>[6x]GSMPLLLDDGDPKAQTGFDLSTATTLFWRPVPVHVKQQDREDV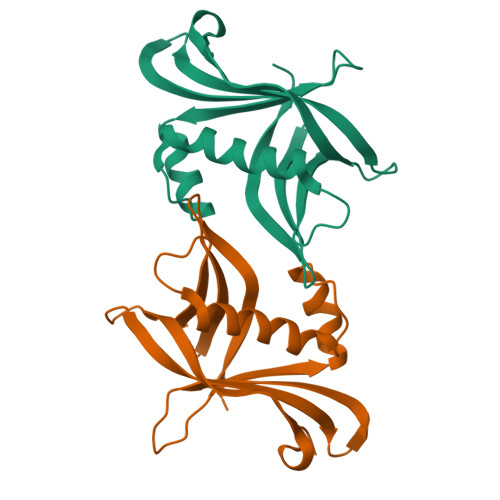LEELTFRILTGVAKQNHNLRILRIHISSDSDLFFLHTLEVSEEDFQSLKNDQGILVDFASFPGKIISLLEKCILAQPGDSPRFQAVLTIRGGESVFKIVEINDFKQLPHITLAFRPGN>SAAPSVFLIDDDRDLRKAMQQTL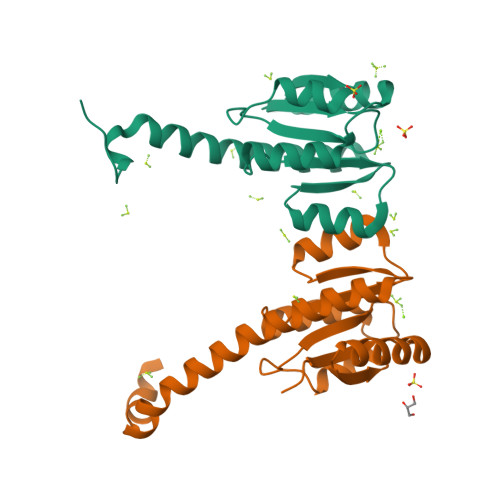ELAGFTVSSFASATEALAGLSADFAGIVISDIRMPGMDGLALFRKILALDPDLPMILVTGHGDIPMAVQAIQDGAYDFIAKPFAADRLVQSARRAEKKRRLVMENRSLRRAAEAASEGLKLAAALEHHHHHH[2x]> GIEETIDTVITNALQLSQPKPQKQPTAQSTPLTSGVNSQEVPALTAVETGASGQAVPSDVIETRHVVNYKTRSESTLESFFGRSACVTILEVENFNATTDADRKKQFTTWAITYTDTVQLRRKLEFFTYSRFDLEMTFVITERYYASNTGHARNQVYQLMYIPPGAPRPTAWDDYTWQSSSNPSVFYTYGSAPPRMSIPYVGIANAYSHFYDGFARVPLKDETVDSGDTYYGLVTINDFGTLAVRVVNEYNPARITSKIRVYMKPKHVRCWCPRPPRAVPYRGEGVDFKQDSITPLTAVENINTF;> SPNVEACGYSDRVRQITLGNSTITTQEAANAVVAYGEWPSYLDDKEANPIDAPTEPDVSSNRFYTLDSVQWKSTSRGWWWKLPDALKDMGMFGQNMYYHYLGRSGYTVHVQCNASKFHQGALGVFAIPEYVMACNTEAKTSYVSYVNANPGEKGGVFDNAYNPSAEASEGRKFAALDYLLGCGVLAGNAFVYPHQIINLRTNNSATLVLPYVNSLAIDCMAKHNNWGLVILPLCKLDYAPNSSTEIPITVTIAPMFTEFNGLRNITVPATQ;> GLPTMLTPGSSQFLTSDDFQSPCALPNFDVTPPIHIPGEVFNMMELAEIDSMIPMNSVTGKANTMEMYPIPLDDKGSATPIFSISLSPASDKRLQYTMLGEILNYYTHWTGSLRFTFLFCGSMMATGKILLSYSPPGAKPPTTRKDAMLGTHIIWDLGLQSSCTMLAPWISNTVYRRCIKDDFTEGGYITCFYQTRIVVPSGTPTSMFMLAFVSACPDFSVRLLRDTNHISQRTLFARAQ;> MGAQVSSQKVGAHENTNVATGGSTVNYTTINYYKDSASNAASKLDFSQDPSKFTEPVKDIMIKTAPALN

Coxsackievirus A24 variant (CVA24v) and enterovirus 70 (EV70) are responsible for several outbreaks of a highly contagious eye disease called acute hemorrhagic conjunctivitis (AHC). However, the AHC-causing human picornaviruses CVA24v and EV70 use glycan-containing receptors for cell attachment. As is typical for picornaviruses, the four capsid proteins (VP1-4) assemble into an icosahedral pseudo T3-capsid. CVA24v recognizes the receptor at a solvent exposed site on the virus shell by interactions with a single capsid protein VP1.

We detected additional difference electron density towards the pentameric VP1 channel in all structures. This electron density does not result from glycan binding and is most likely a remainder of the virus preparation, as it is observed in a different crystal form (CVA24v-acidic).> SNAMKISKVREENRGAKLTVNAKTAVVSENRSQEGILYNDPSRYGKSRKNDEDRDRYIESRLKSSGKLYRIFNEDKNKRETDELQWFLSEIVKKINRRNGLVLSDMLSVDDRAFEKAFEKYAELSYTNRRNKVSGSPAFETCGVDAATAERLKGIISETNFINRIKNNIDNKVSEDIIDRIIAKYLKKSLCRERVKRGLKKLLMNAFDLPYSDPDIDVQRDFIDYVLEDFYHVRAKSQVSRSIKNMNMPVQPEGDGKFAITVSKGGTESGNKRSAEKEAFKKFLSDYASLDERVRDDMLRRMRRLVVLYFYGSDDSKLSDVNEKFDVWEDAAARRVDNREFIKLPLENKLANGKTDKDAERIRKNTVKELYRNQNIGCYRQAVKAVEEDNNGRYFDDKMLNMFFIHRIEYGVE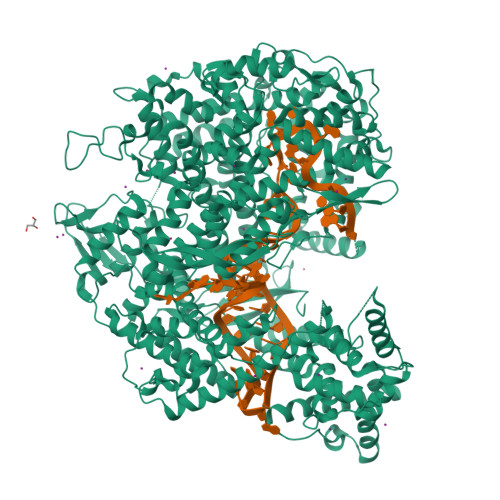KIYANLKQVTEFKARTGYLSEKIWKDLINYISIKYIAMGKAVYNYAMDELNASDKKEIELGKISEEYLSGISSFDYELIKAEEMLQRETAVYVAFAARHLSSQTVELDSENSDFLLLKPKGTMDKNDKNKLASNNILNFLKDKETLRDTILQYFGGHSLWTDFPFDKYLAGGKDDVDFLTDLKDVIYSMRNDSFHYATENHNNGKWNKELISAMFEHETERMTVVMKDKFYSNNLPMFYKNDDLKKLLIDLYKDNVERASQVPSFNKVFVRKNFPALVRDKDNLGIELDLKADADKGENELKFYNALYYMFKEIYYNAFLNDKNVRERFITKATKVADNYDRNKERNLKDRIKSAGSDEKKKLREQLQNYIAENDFGQRIKNIVQVNPDYTLAQICQLIMTEYNQQNNGCMQKKSAARKDINKDSYQHYKMLLLVNLRKAFLEFIKENYAFVLKPYKHDLCDKADFVPDFAKYVKPYAGLISRVAGSSELQKWYIVSRFLSPAQANHMLGFLHSYKQYVWDIYRRASETGTEINHSIAEDKIAGVDITDVDAVIDLSVKLCGTISSEISDYFKDDEVYAEYISSYLDFEYDGGNYKDSLNRFCNSDAVNDQKVALYYDGEHPKLNRNIILSKLYGERRFLEKITDRVSRSDIVEYYKLKKETSQYQTKGIFDSEDEQKNIKKFQEMKNIVEFRDLMDYSEIADELQGQLINWIYLRERDLMNFQLGYHYACLNNDSNKQATYVTLDYQGKKNRKINGAILYQICAMYINGLPLYYVDKDSSEWTVSDGKESTGAKIGEFYRYAKSFENTSDCYASGLEIFENISEHDNITELRNYIEHFRYYSSFDRSFLGIYSEVFDRFFTYDLKYRKNVPTILYNILLQHFVNVRFEFVSGKKMIGIDKKDRKIAKEKECARITIREKNGVYSEQFTYKLKNGTVYVDARDKRYLQSIIRLLFYPEKVNMDEMIEVKEKKKPSDNNTGKGYSKRDRQQDRKEYDKYKEKKKKEGNFLSGMGGNINWDEINAQLKN> EWKQGTEAAAVRSGDKVFFAGDSLMQGVAPFVQKSLKQQYGIESANLSKQSTGLSYPSFFDWPKTIEETLKKHPEISVLAVFLGPNDPWDFPVGKRYLKFASDEWAQEYLKRVDRILEAAHTHRVQVVWLGIPYMKKVKLDGQMRYLDKLLSEHLKGKIILIPTAQTLSGGKGRYTDSVNVNGKPVRYRSKDGIHFTAEGQKLLAEKIMEKIVF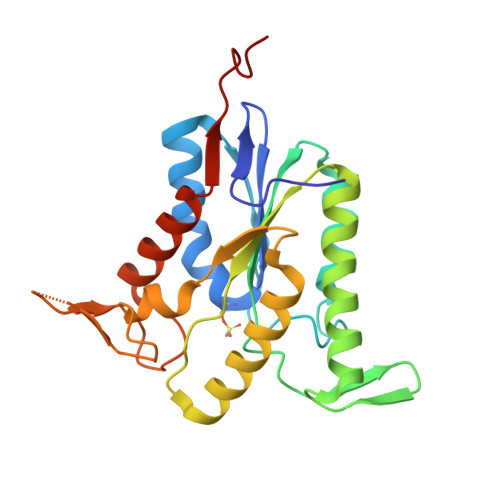EPSTQPSSTQP In human mitochondria, mitochondrial Hsp70 (mortalin) and the nucleotide exchange factor (GrpEL1) work synergistically to stabilize proteins, assemble protein complexes, and facilitate protein import. In bacteria, mitochondria, and chloroplasts, the GrpE-family of NEFs interacts with substrate-bound Hsp70 to facilitate ADP and protein substrate release. Herein, we present structures of full-length human mortalin in a nucleotide-free and substrate-bound state in complex with full-length GrpEL1. To stabilize the complex for structural analysis, we introduced a point mutation, R126W, into mortalin (mortalinR126W) that is associated with EVEN-PLUS syndrome and has been shown to reduce mortalin’s ATPase activity and conformational flexibility.

Thus, we mutated Y173 in GrpEL1 to an alanine (GrpEL1Y173A) and performed cryoEM analysis on a mortalinR126W-GrpEL1Y173A complex. Our cryoEM analysis of mortalinR126W-GrpEL1Y173A yielded two distinct populations differentiated by the presence or lack of density for the SBDα lid. We term these structures mortalinR126W-GrpEL1Y173A and mortalinR126W-GrpEL1Y173A−lid. Overall, these structures closely resemble our mortalinR126W-GrpEL1WT structure and are similarly nucleotide-free. In our mortalinR126W-GrpEL1Y173A−lid structure, we discern diminished EM density for the IDL region and density only for the SBDβ subdomain. Importantly, we are unable to identify EM density of bound substrate that is observed in our other mortalinR126W-GrpEL1 structures. Considering density for the SBDα subdomain is also absent in the mortalinR126W-GrpEL1Y173A−lid structure, we hypothesize that this complex harbors a disordered SBDα subdomain and may represent a post-substrate release state. Finally, the lack of SBDα density in our mortalinR126W-GrpEL1Y173A−lid structure suggests flexibility of the SBDα lid, especially in the absence of substrate.

> MASEAIKGAVVGIDLGTTNSCVAVMEGKQAKVLENAEGARTTPSVVAFTADGERLVGMPAKRQAVTNPNNTFYATKRLIGWRYDDPEVQKDIKNVPFKIVRASNGDAWVEAHGKLYSPSQIGAFVLMKMKETAENYLGHTAKNAVITVPAYFNDSQRQATKDAGQISGLNVLRVINEPTAAALAYGLDKSEDKVIAVYDLGGGTFDISILEIQKGVFEVKSTNGDTFLGGEDFDQALLRHIVKEFKRETGVDLTKDNMALQRVREAAEKAKCELSSSVQTDINLPYLTMDSSGPKHLNMKLTRAQFEGIVTDLIRRTIAPCQKAMQDAEVSKSDIGEVILVGGMTRMPKVQQTVQDLFGRAPSKAVNPDEAVAIGAAIQGGVLAGDVTDVLLLDVTPLSLGIETLGGVFTKLINRNTTIPTKKSQVFSTAADGQTQVEIKVCQGEREMAGDNKLLGQFTLIGIPPAPRGVPQIEVTFDIDANGIVHVSAKDKGTGREQQIVIQSSGGLSKDDIE;>[2x]TLLEEKVKLEEQLKETVEKYKRALADTENLRQRSQKLVEEAKLYGIQAFCKDLLEVADVLEKATQCVPKEEIKDDNPHLKNLYEGLVMTEVQIQKVFTKHGLLKLNPVGAKFDPAEHEALFHTPVEGKEPGTVALVSKVGYKLHGRTLRPALVGVVKEASA> GTLTGERPPVFWLQGQGCTGCSVTLLNSVHPSIADVLLKVISLEFHPTVMAWEGEHAIEHMRKVAEKFKGKFFLVIEGSVPVEADGKYCIIGEANHHEISMVDALKEFGPNAAAVLAVGTCAAYGGIPAAEGSETGATAVSKFLGDNGIKTPVVNIPGCPPHPDWIVGTVVLALDAIKKNGLEGGLAEVVKVLDSDGRPTPFFGRNIHENCPYLDKYDEGVMSATFTDKVGCRYDLGCKGPMTMADCFERKWNGGVNWCVQNAVCIGCVEPDFPDGKSPFYQA;> GATGRTTIAIDPVTRIEGHLKAEVVVENGKVVDARLSGGMYRGFETILRGRDPRDASQIVQRICGVCPTAHSTASVLALDEAFGAKVPNNGRITRNLIFGANYLQSHILHFYH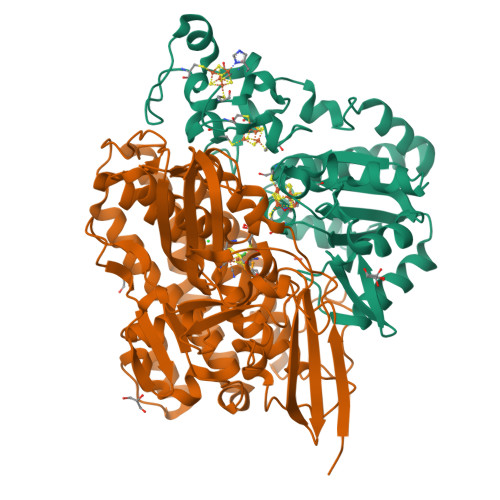LSAQDFVQGPDTAPFVPRFPKSDLRLSKELNKAGVDQYIEALEVRRICHEMVALFGGRMPHVQGQVVGGATEIPTKEKLVEYAARFKKVRDFVEQKYVPVVYTIGSKYKDMFKVGQGFKAALCVGAFPLDNSGKKHLFMPGVYAKGKDMPFDPSKIKEYVKYSWFAEETTGLNYKEGKTIPAPDKAGAYSFVKAPRYDGLSLEVGPLARMWVNNPELSPVGKKLLKDLFGISAKKFRDLGEEAAFSLMGRHVARAEETYYMLGAIEGWLKEIKAGEDTVVMPAVPASAEGTGFTEAPRGSLLHYVKVKDSKIDNYQIVSASLWNCNPRDDMGQRGAVEEALIGIPVDDIQNPVNVARLIRAFDPULSCAVH> MSIDSALNWDGEMTVTRFDSKTGAHFVIRLDSTQLGPAAGGTRAAQYSQLADALTDAGKLAGAMTLKMAVSNLPMGGGKSVIALPAPRHSIDPSTWARILRIHAENIDKLSGNYWTGPDVNTNSADMDTLNDTTEFVFGRSLERGGAGSSAFTTAVGVFEAMKATVAHRGLGSLDGLTVLVQGLGAVGGSLASLAAEAGAQLLVADTDTERVAHAVALGHTAVALEDVLSTPCDVFAPCAMGGVITTEVARTLDCSVVAGAANNVIADEAASDILHARGILYAPDFVANAGGAIHLVGREVLGWSESVVHERAVAIGDTLNQVFEISDNDGVTPDEAARTLAGRRARE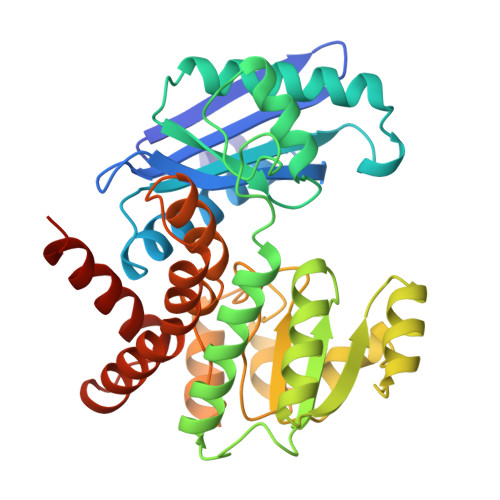ASTTTATA> MESLPVIAAPSMWTRPQIKDFKEKIRQDADSVITVGRGEVVTVRVPTHEEGSYLFWEFATDNYDIGFGVYFEWTDSPNTAVSVHVSESSDDDEEEEENISSEEKAKKNANKPLLDEIVPVYRRDCHEEVYAGSHQY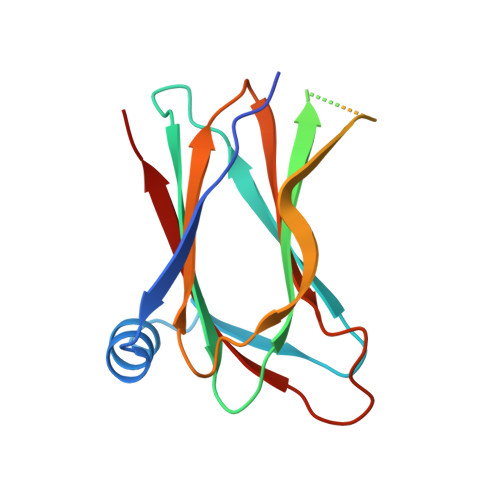PGRGVYLLKFDNSYSLWRSKSVYYRVYYTR> APVRSLNCRIWDVNQKTFYLRNNQLVAGYLQGPNVNLEEKFSMSFVQGEESNDKIPVALGLKEKNLYLSCVLKDDKPTLQLESVDPKNYPKKKMEKRFVFNKIEINNKLEFESAQFPNWFLCTAMEADQPVSLTNMPDEGVMVTKFYMQFVSS;> LEADKCKEREEKIILVSSANEIDVRPCPLNPNEHKGTITWYKDDSKTPVSTEQASRIHQHKEKLWFVPAKVEDSGHYYCVVRNSSYCLRIKISAKFVENEPNLCYNAQAIFKQKLPVAGDGGLVCPYMEFFKNENNELPKLQWYKDCKPLLLDNIHFSGVKDRLIVMNVAEKHRGNYTCHASYTYLGKQYPITRV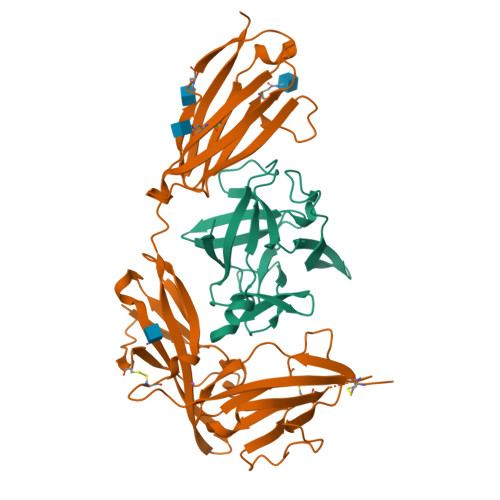IEFITLEENKPTRPVIVSPANETMEVDLGSQIQLICNVTGQLSDIAYWKWNGSVIDEDDPVLGEDYYSVENPANKRRSTLITVLNISEIESRFYKHPFTCFAKNTHGIDAAYIQLIYPVTNFQK>[2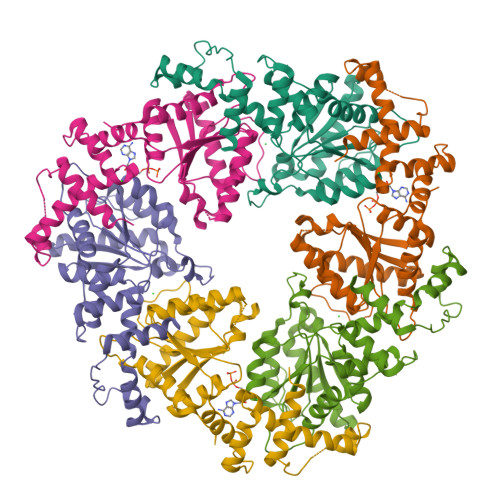x]SYYIAPRFLDKLAVHITKNFLNIPGVRVPLILGIHGRKGEGKTFQCELAFEKMGIEVTLISGGELESPDAGDPARLIRLRYRETAELIKVRGKMCVLMINDLDAGAGRFDEGTQYTVNTQLVNATLMNIADNPTDVQLPGSYDSNPIRRVPIIVTGNDFSTLYAPLIRDGRMEKFYWEPNRDDKVGIVGGIFAEDGLSQREIEQLVDTFPKQSIDFFSALRSRIYDIQIRDFIHKVGFERISLRVVNSLEAPPEFKKPDFSLAHLIESGNLVLGEQQRVDNSQLVDEYNR>MQIGFNFTLTGTLDMVQQMIKERKIDYVEMLIDNFVHLPPEQIADSFDCPVAFHIMLSKYLERDREALAALGKRLRRFIDVMRPVYVSDHILYFTHNGRSLFHLGEIDYGEYDHVRSKVEQWQDMLGTRLYLENYPSIMDGAWDAPSFYERLSRETGVGVLFDASNAICAQNNTGAPVELWKKIIETTRHFHVAGYGTAFIEPRVKADTHDREMAEDTLDFLSRMRTSFDKPGATITYERDFDIDYESISVDLKRLRDIFPCVEEERH[2x];>[2x]MSLLPTAPVRID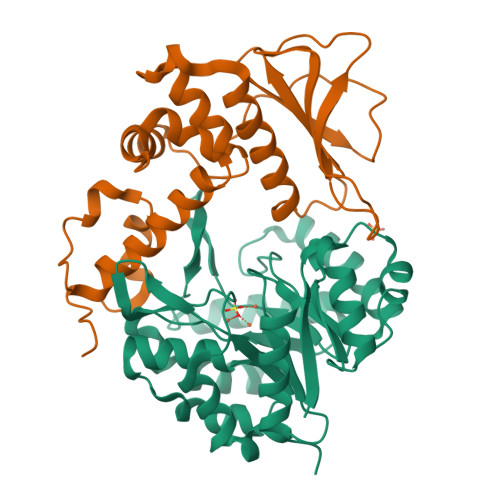ADLYDDLANPARQSLYPRDSRGFIRIDISLRAYWHTLFDTCPRLLELSGPSGGAIFLPFMAWARENNLAFDWSFFLWVYVWLQQSEFRERLDEDQLLPVMTASATRWLMIDRDIDACQIVLGSRSLAGAAVVGAKIDSIHCRLEQVQQVAFAAPLPLPDGEFGYFLTPGFEIDHFPGWRPLPR> SLQLWQFLVALLDDPSNSHF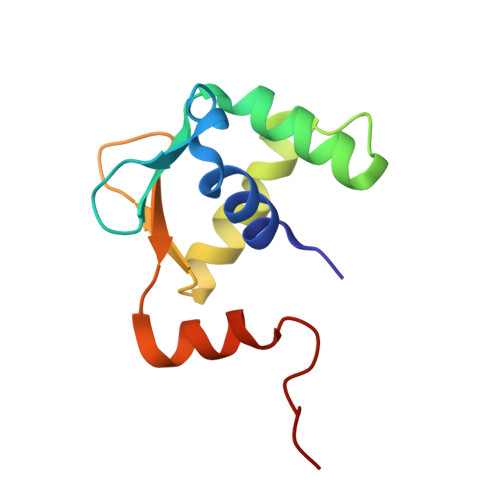IAWTGRGMEFKLIEPEEVARRWGIQKNRPAMNYDKLSRSLRYYYEKGIMQKVAGERYVYKFVCDPEALFSMAFPDNQRPLL>GPHMTQEEAVVNASLWEYVRLRESYDADTAQYAYDLVSNFSAPMVRQNYQQFFNYPNPTSPQVILGKHGRLEVEHIASNDVTPGVQQIRYKRTLIVDGKMPMASTWTATVRYEKVTSLPGRLRLTNPGGLVVTSYQTSEDTVSN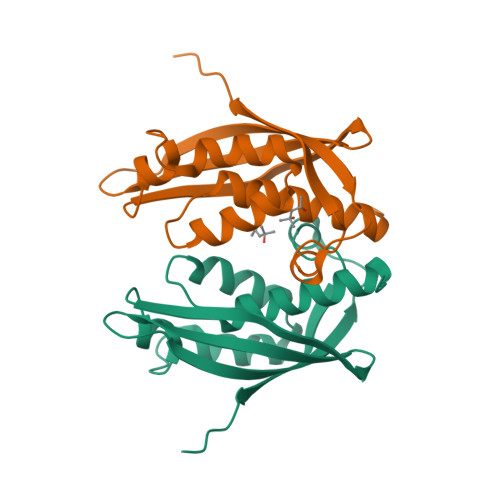AGHSEP[2x]> MSSNRVLDLFKPFESFLPEVIAPERKVPYNQKLIWTGVSLLIFLILGQIPLYGIVSSETSDPLYWLRAMLASNRGTLLELGVSPIITSSMIFQFLQGTQLLQIRPESKQDRELFQIAQKVCAIILILGQALVVVMTGNYGAPSDLGLPICLLLIFQLMFASLIVMLLDELLSKGYGLGSGISLFTATNIAEQIFWRAFAPTTVNSGRGKEFEGAVIAFFHLLAVRKDKKRALVEAFYRTNLPNMFQVLMTVAIFLFVLYLQGFRYELPIRSTKVRGQIGIYPIKLFYTSNTPIMLQSALTSNIFLISQILFQKYPTNPLIRLIGVWGIRPGTQGPQMALSGLAYYIQPLMSLSEALLDPIKTIVYITFVLGSCAVFSKTWIEISGTSPRDIAKQFKDQGMVINGKRETSIYRELKKIIPTAAAFGGATIGALSVGSDLLGTLGSGASILMATTTIYGYYEAAAKEGGFTKNLVPGFSDLM;> MSSPTPPGGQRTLQKRKQGSSQKVAASAPKKNTNSNNSILKIYSDEATGLRVDPLVVLFLAVGFIFSVVALHVISKVAGKLF;> MARASEKGEEKKQSNNQVEKLVEAPVEFVREGTQFLAKCKKPDLKEYTKIVKAVGIGFIAVGIIGYAIKLIHIPIRYVIV;> MPTNYEYDEASETWPSFILTGLLMVVGPMTLLQIYQIFFGANAEDGNSGKSKEFNEEVFKNLNEEYTSDEIKQFRRKFDKNSNKKSKIWSRRNIIIIVGWILVAILLQRINSNDAIKDAATKLFDPYEILGISTSASDRDIKSAYRKLSVKFHPDKLAKGLTPDEKSVMEETYVQITKAYESLTDELVRQNYLKYGHPDGPQSTSHGIALPRFLVDGSASPLLVVCYVALLGLILPYFVSRWWARTQSYTKKGIHNVTASNFVSNLVNYKPSEIVTTDLILHWLSFAHEFKQFFPDLQPTDFEKLLQDHINRRDSGKLNNAKFRIVAKCHSLLHGLLDIACGFRNLDIALGAINTFKCIVQAVPLTPNCQILQLPNVDKEHFITKTGDIHTLGKLFTLEDAKIGEVLGIKDQAKLNETLRVASHIPNLKIIKADFLVPGENQVTPSSTPYISLKVLVRSAKQPLIPTSLIPEENLTEPQDFESQRDPFAMMSKQPLVPYSFAPFFPTKRRGSWCCLVSSQKDGKILQTPIIIEKLSYKNLNDDKDFFDKRIKMDLTKHEKFDINDWEIGTIKIPLGQPAPETVGDFFFRVIVKSTDYFTTDLDITMNMKVRDSPAVEQVEVYSEEDDEYSTDDDETESDDESDASDYTDIDTDTEAEDDESPE;> MSEFNETKFSNNGTFFETEEPIVETKSISVYTPLIYVFILVVSLVMFASSYRKKQAKKISEQPSIFDENDAHDLYFQIKEMSENEKIHEKVLKAALLNRGAESVRRSLKLKELAPQINLLYKNGSIGEDYWKRFETEVKLIELEFKDTLQEAERLQPGWVQLFVMVCKEICFNQALSRRYQSILKRKEVCIKEWELKINNDGRLVN;> MVTLEYNANSKLITASDAVVALSTETNIDQINVLTTSLIGETNPNFTPQPNEALSKMIKGLFESGMKNLQQKKLNEALKNVSLAIEMAQRKRAPWEAFAIQLPELHFMLRSK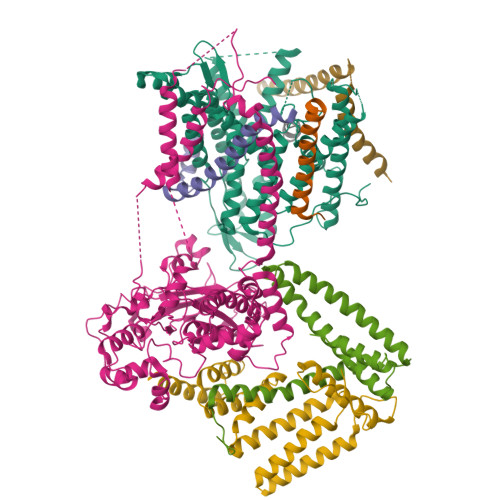IDLCLILGKHLEALQDLDFLLGTGLIQPDVFVRKADCLLKLRQWEEARATCERGLALAPEDMKLRALLIETARNLAEYNGE;> MSAVGPGSNAGASVNGGSATAIATLLRNHKELKQRQGLFQAKQTDFFRYKRFVRALHSEEYANKSARQPEIYPTIPSNKIEDQLKSREIFIQLIKAQMVIPVKKLHSQECKEHGLKPSKDFPHLIVSNKAQLEADEYFVWNYNPRTYMDYLIVIGVVSIILALVCYPLWPRSMRRGSYYVSLGAFGILAGFFAVAILRLILYVLSLIVYKDVGGFWIFPNLFEDCGVLESFKPLYGFGEKDTYSYKKKLKRMKKKQAKRESNKKKAINEKAEQNXXXXXXXXXXXXXXXXXXXXXXXXXXXXXXXXXXXXXXXXXXXXXXXXXX;> MRFPSIFTAVLFAASSALAAPVNTTTEDETAQIPAEAVIGYLDLEGDFDVAVLPFSNSTNNGLLFINTTIASIAAKEEGVSLDKREAEAWHWLQLKPGQPMYKREAEAEAWHWLQLKPGQPMYKREADAEAWHWLQLKPGQPMYKREADAEAWHWLQLKPGQPMYXXXXXXXXXXXXX>[2x]MDSVDVVVIGGGQSGLSAGYFLRRSGLSYVILDAEASPGGAWQHAWHSLHLFSPAGWSSIPGWPMPASQGPYPARAEVLAYLAQYEQKYAL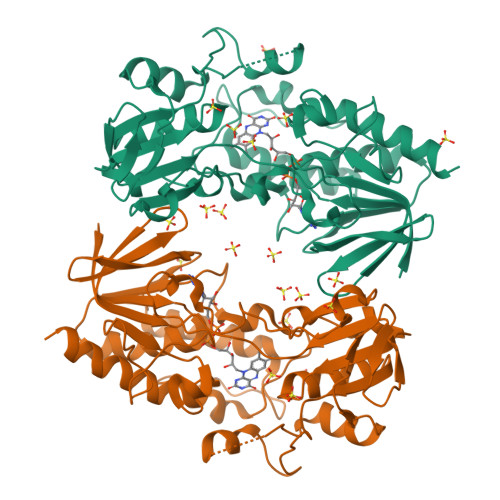PVLRPIRVQRVSHFGERLRVVARDGRQWLARAVISATGTWGEAYTPEYQGLESFAGIQLHSAHYSTPAPFAGMRVAIIGGGNSGAQILAEVSTVAETTWITQHEPAFLADDVDGRVLFERATERWKAQQEGREPDLPPGGFGDIVMVPPVLDARARGVLAAVPPPARFSPTGMQWADGTERAFDAVIWCTGFRPALSHLKGLDLVTPQGQVEVDGSGLRALAVPSVWLLGYGDWNGMASATLIGVTRYAREAVRQVTAYCADHQDR> GSGGSIRLADLAQQLDAELHGDGDIVITGVASMQSAQTGHITFMVNPKYREHLGLCQASAVVMTQDDLPFAKSAALVVKNPYLTYARMAQILDTTPQPAQNIAPSAVIDATAKLGNNVSIGANAVIESGVELGDNVIIGAGCFVGKNSKIGAGSRLWANVTIYHEIQIGQNCLIQSGTVVGADGFGYANDRGNWVKIPQIGRVIIGDRVEIGACTTIDRGALDDTIIGNGVIIDNQCQIAHNVVIGDNTAVAGGVIMAGSLKIGRYCMIGGASVINGHMEICDKVTVTGMGMVMRPITEPGVYSSGIPLQPNKVWRKTAALV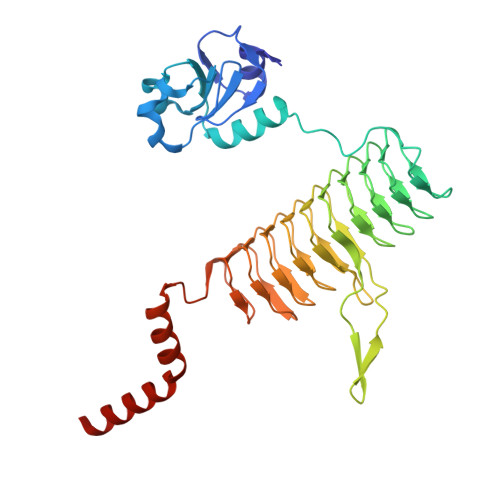MNIDDMSKRLKSLERKVNQQD>[2x]HMGSDTDE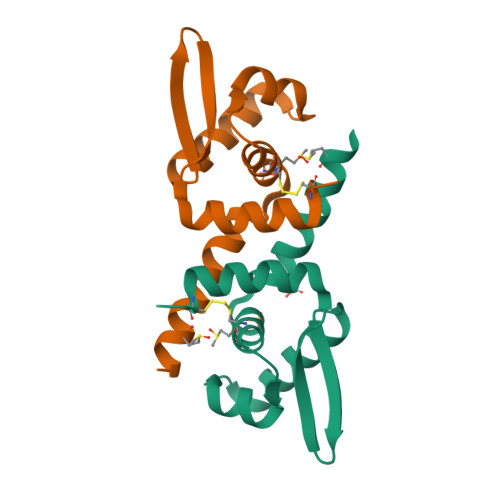RSAALDAEEMATRARAASNLLKALAHEGRLMIMCYLASGEKSVTELETRLSTRQAAVSQQLARLRLEGLVQSRREGKTIYYSLSDPRAARVVQTVYEQFCSGD>SSLKPFTYPFPETRFLHAGPNVYKFKIRYGKSIRGEEIENKEVITQELEDSVRVVLGNLDNLQPFATEHFIVFPYKSKWERVSHLKFKHGEIILIPYPFVFTLYVEMKW[3x];>TGYISIDAMKKFLGELHDFIPGTSGYLAYHVQNEIN[3x]

TERB1 is a molecular scaffold that simultaneously interacts with TERB2 and shelterin subunit TRF1. Knockout of any components of the TERB1–TERB2–MAJIN (TTM) complex impairs the telomere–NE attachment and results in infertility in both male and female mice. In the present study, we characterize the TERB1–TERB2 and TERB2–MAJIN interactions and determine the crystal structures of the N-terminal domains of TERB2 and MAJIN in complex with TERB2-binding motif of TERB1 and MAJIN-binding motif of TERB2, respectively. To reveal the structural basis for the interactions between TERB1 and TERB2 and between TERB2 and MAJIN, we crystallized the TERB1587–659–TERB22–116 and the TERB2119–220–MAJIN2–149 complexes and determined their structures using single-wavelength anomalous dispersion (SAD) method at resolutions of 3.3 and 2.9 Å, respectively.

Our data revealed that a short fragment of TERB2 at the C-terminus (residues 168–202) is sufficient for interaction with MAJIN. In the TERB2MBM-MAJINNTD complex, MAJINNTD adopts a compact fold with a curved four-stranded β sheet (β1–β2–β3–β5) holding helix α1 in the center. The TERB2MBM polypeptide forms an extended structure that wraps around the surface of MAJINNTD. The driving force for the binding of TERB2MBM to MAJINNTD is van der Waals interactions. The highly hydrophobic TERB2MBM polypeptide meanders along a hydrophobic groove on the surface of MAJINNTD and buries a total of ∼1300 Å2 surface area at the interface. The C-terminus of TERB2MBM and the loop between strands β3 and β5 of MAJINNTD contact each other and fold into an intermolecular anti-parallel β sheet that packs onto the central β sheet of MAJINNTD to further strengthen the interaction. It is worthy of noticing that, although there are three TERB2MBM–MAJINNTD complexes in one asymmetric unit in the crystal structure, two protomer complexes apparently form a heterotetramer with an extensive hydrophobic dimeric interface between two MAJINNTD molecules. Consistent with a recent study, this observation suggests that TERB2 and MAJIN could form a heterotetramer with a 2:2 stoichiometry. In particular, located at the center of this interface, the side chain of Phe192 of TERB2 is buried in a pocket formed by a group of hydrophobic residues of both MAJIN and TERB2. Again consistent with the crystal structure, substitution of Phe192TERB2 with a negatively charged bulk arginine residue completely abolished the TERB2–MAJIN interaction in 293T cells.> MADLKAAEVEKAREHFEIYDWEGEGKIDARDLGDLLRSLDCKPTLAMVKKNGGSDKRGEKKLTLEEFLPIFSQIKKEKEVGTLEDFMEGLKVYDKA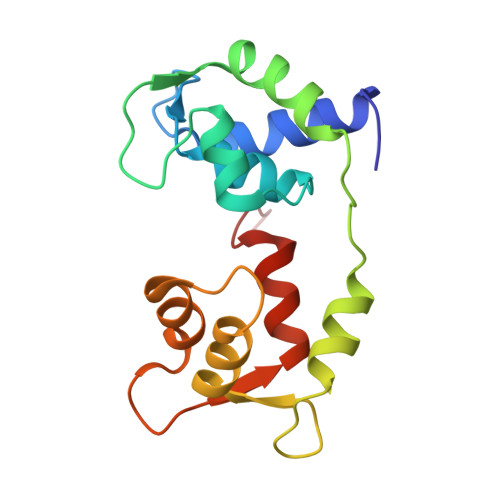ENGTMLAAELAHVLLSLGERLTDIECEEIMRVCDEDDDGFLKYEPFVKTIIAGPFPDEGK> MIKLKNVTKTYKMGEEIIYALKNVNLNIKEGEFVSIMGPSGSGKSTMLNIIGCLDKPTEGEVYIDNIKTNDLDDDELTKIRRDKIGFVFQQFNLIPLLTALENVELPLIFKYRGAMSGEERRKRALECLKMAELEERFANHKPNQLSGGQQQRVAIARALANNPPIILADEPTGALDSKTGEKIMQLLKKLNEEDGKTVVVVT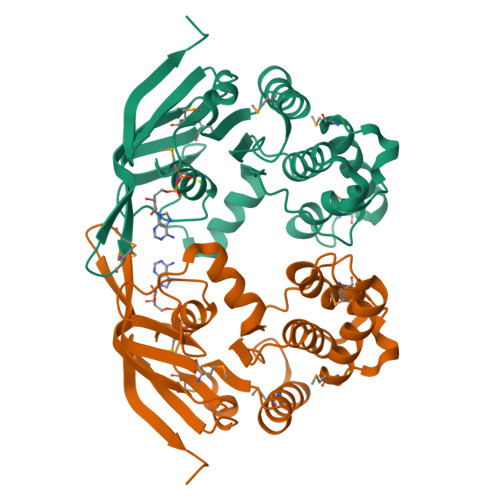HDINVARFGERIIYLKDGEVEREEKLRGFDDR(2~{S})-~{N}-[(1~{R},2~{S})-1-cyano-1-oxidanyl-3-[(3~{S})-2-oxidanylidenepiperidin-3-yl]propan-2-yl]-3-phenyl-2-[[(~{E})-3-phenylprop-2-enoyl]amino]propanamide | C27 H30 N4 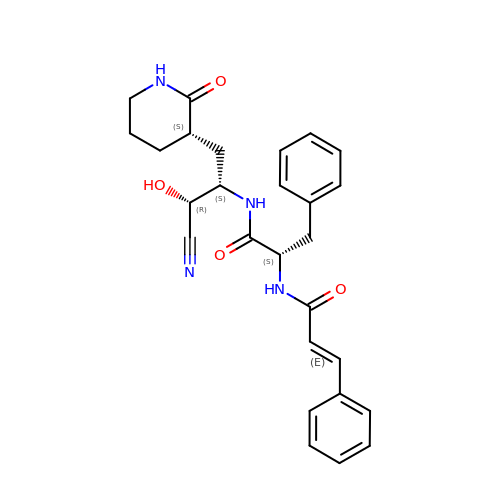O4 | UJFNOZFDUMAJFU-XSAZPJIKSA-N> SKTAKIDWSHWTVTVPEENPDKPGKPYSLGYPEILNYAEDKIASKYMYDDPKDKSVVFYAFPSGVTTANTHYSRSELRETMETGSNKVNWTFAKGGKMRGTYAIDDISKEPDGKYSRVIIAQIHGV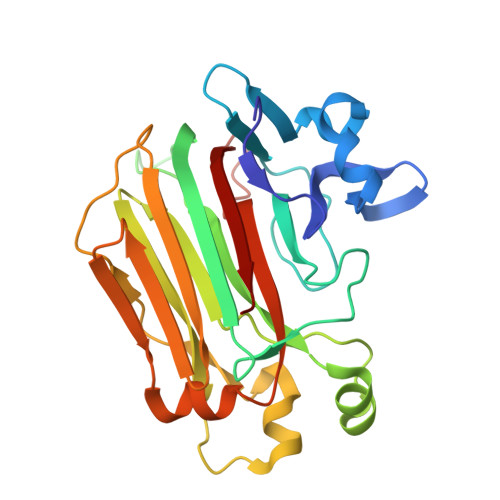LTDEQRDLIGQKDNNAPPILKVYWDKGKIRVKTKVLKDLNAPYKEMLSEDAWGDDEGRNFKEKIDLNTRFTLEVKVSDGRMEVILNDTESLVYDDIHMKKWGIFENYFKAGNYFQSKTPGTFAKVKIYSLQVTHL> GAMAAGTLYTYPENWRAFKALIAAQYSGAQVRVLSAPPHFHFGQTNRTPEFLRKFPAGKVPAFEGDDGFCVFESNAIAYYVSNEELRGSTPEAAAQVVQWVSFADSDIVPPASTWVFPTLGIMHH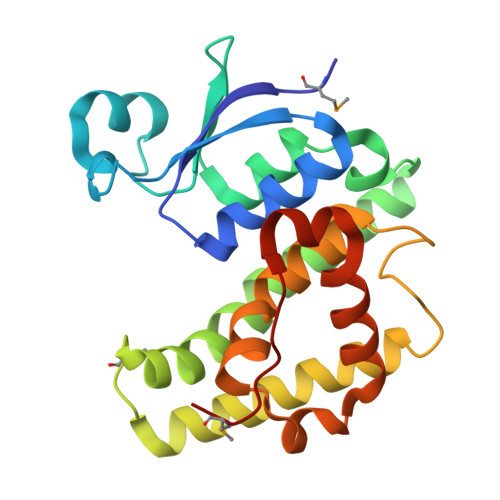NKQATENAKEEVRRILGLLDAYLKTRTFLVGERVTLADITVVCTLLWLYKQVLEPSFRQAFPNTNRWFLTCINQPQFRAVLGEVKLCEKMAQFDA> AAMAFTLADRVTEEMLADKAALVVEVVEENYHDAPIVGIAVVNEHGRFFLRPETALADPQFVAWLGDETKKKSMFDSKRAAVALKWKGIELCGVSFDLLLAAYLLDPAQGVDDVAAAAKMKQYEAVRPDEAVYGKGAKRAVPDEPVLAEHLVRKAAAIWELERPFLDELRRNEQDRLLVELEQPLSSILAEMEFAGVKVDTKRLEQMGKELAEQLGTVEQRIYELAGQEFNINSPKQLGVILFEKLQLPVLKKTKTGYSTSADVLEKLAPYHEIVENILHYRQLGKLQSTYIEGLLKVVRPDTKKVHTIFNQALTQTGRLSSTEPNLQNIPIRLEEGRKIRQAFVPSESDWLIFAADYSQIELRVLAHIAEDDNLMEAFRRDLDIHTKTAMDIFQVSEDEVTPNMRRQAKAVNFGIVYGISDYGLAQNLNISRKEAAEFIERYFESFPGVKRYMENIVQEAKQKGYVTTLLHRRRYLPDITSRNFNVRSFAERMAMNTPIQGSAADIIKKAMID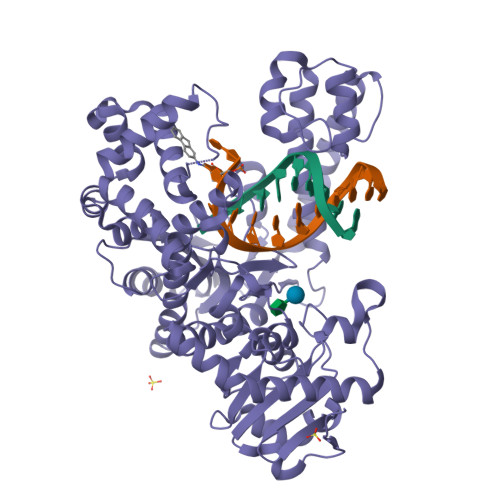LNARLKEERLQAHLLLQVHDELILEAPKEEMERLCRLVPEVMEQAVTLRVPLKVDYHYGSTWYDAK The Arabidopsis VEL proteins are accessory proteins that interact with PRC2 to nucleate and propagate silencing at the FLOWERING LOCUS C (FLC) locus, enabling early flowering in spring. Here, we report that VEL proteins contain a domain related to an atypical four-helix bundle that engages in spontaneous concentration-dependent head-to-tail polymerization to assemble dynamic biomolecular condensates. The VEL domain adopts a compact globular fold, consisting of four α-helices in a quasi-antiparallel “up-down-up-down” configuration, each of which contributes to the hydrophobic core, as illustrated by VEL1VEL. Mutations blocking polymerization of this VEL domain prevent Polycomb silencing at FLC.

We conclude that the VEL head and tail surfaces are defined largely by three key residues, an isoleucine (VIN3I575 or VEL1I664) and two basic residues (VIN3R554,R556 or VEL1R643,K645), that engage in close hydrophobic or electrostatic interactions, respectively, with partner residues from the apposing complementary surface. The equivalent double mutation of VEL1VEL (RK>AD) also essentially blocks polymerization. Importantly, the RK>AD mutant never forms floaters nor fibers.

>[4x]GGTESGLEHCVKIIRQLECSGHIDKNFAQDFLTWYSLRATSQEIRVVKDFIDTFIDDPMALAEQLIDTFDDRVSIKR>[3x]MKKLLPILIGLSLSGFSSLSQAENLMQVYQQARLSNPELR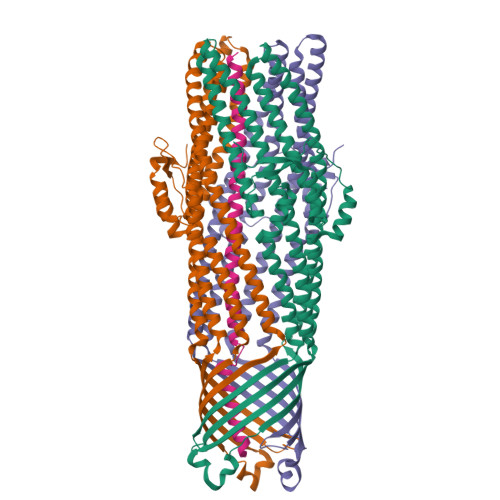KSAADRDAAFEKINEARSPLLPQLGLGADYTYSNGYRDANGINSNATSASLQLTQSIFDMSKWRALTLQEKAAGIQDVTYQTDQQTLILNTATAYFNVLNAIDVLSYTQAQKEAIYRQLDQTTQRFNVGLVAITDVQNARAQYDTVLANEVTARNNLDNAVEQLRQITGNYYPELAALNVENFKTDKPQPVNALLKEAEKRNLSLLQARLSQDLAREQIRQAQDGHLPTLDLTASTGISDTSYSGSKTRGAAGTQYDDSNMGQNKVGLSFSLPIYQGGMVNSQVKQAQYNFVGASEQLESAHRSVVQTVRSSFNNINASISSINAYKQAVVSAQSSLDAMEAGYSVGTRTIVDVLDATTTLYNAKQELANARYNYLINQLNIKSALGTLNEQDLLALNNALSKPVSTNPENVAPQTPEQNAIADGYAPDSPAPVVQQTSARTTTSNGHNPFRN;> METAVAYYKDGVPYDDKGQVIITLLNGTPDGSGSGGGGGKGGSKSESSAAIHATAKWSTAQLKKTQAEQAARAKAAAEAQAKAKANRDALTQRLKDIVNEALRHNASRTPSATELAHANNAAMQAEDERLRLAKAEEKARKEAEAAEKAFQEAEQRRKEIEREKAETERQLKLAEAEEKRLAALSEEAKALEHHHHHH>[2x]GMSLKSTTSSLTTNNHDKTINSVQSLVNGTGTVADHNPYDEVPYESYPYAITNPYHLSTLATLFGINAPEVENSKILELGCAAGGNLIPHAVLYPNAHFVGVDLSKVQIDEANKNVRALGLKNIEFHHCSITDIDDSFGKFDYIICHGVISWVPKIVRDKIFKVCNRNLSTNGIAYISYNTLPGWNMVRTIRDMMLYHSSSFTNIRDRIAQSRLLLEFVKDSLEHSKTPYAEVLKTEAGLLAKQTDHYLRHDHLEEENAQFYFHEFMNEARKHNLQYLADCNISTMYLGNMPPKVVEQLKAVNDIVRTEQYMDFITNRRFRTTLLCHNDLKINRNINNDDIKKFNIIFNVIPEKPLKEVDLNNATENLQFFLNGNKESNLSTTSPYMKAILYTFSENLNNPLSFKQVTSEANTKLNNTKLNEIKNELLNNAMKLVLQGYISITNQKHRSKPVLDKPKTTQMVIYQAKYTPSMWVTNLK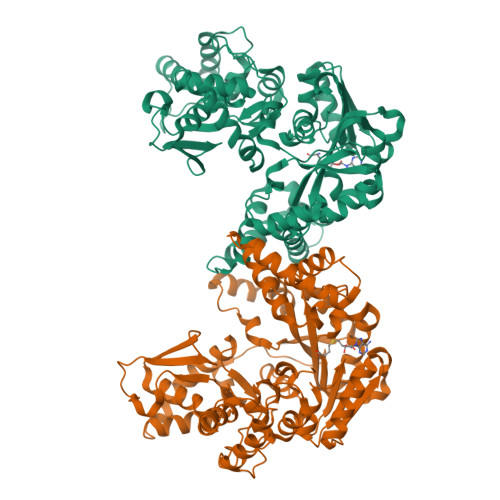HEPIGVNFFEKFALRYMDGRNDKKAIIEAILGHVEKGELTLSREGQKIENKEEIRKELESLFTPMIEKFCSNALLV6-ethyl-1-oxidanylidene-indene-4-carboxylic 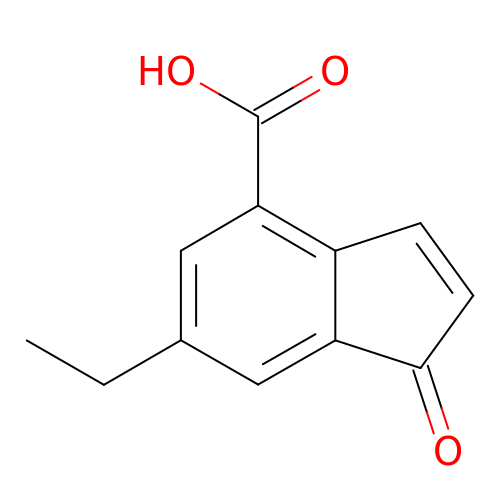acid | C12 H10 O3 | XWFSVEPQDLTABF-UHFFFAOYSA-N1-[[3-(aminomethyl)phenyl]methyl]-2-butyl-imidazo[4,5-c]quinolin-4-amine | C22 H25 N5 | 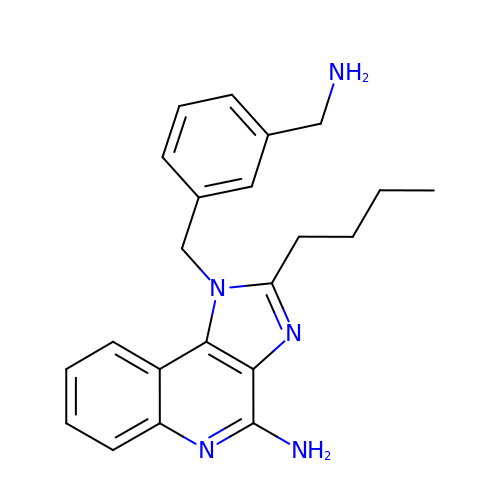AKLBWCHTGHQPMA-UHFFFAOYSA-N> GPLHMKAVVPGPA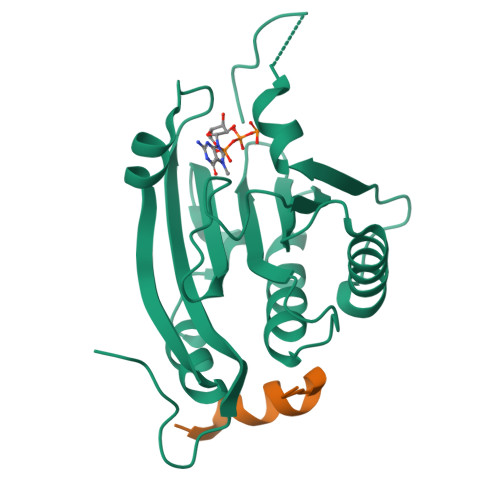EHPLQYNYTFWYSRRTPGRPTSSQSYEQNIKQIGTFASVEQFWRFYSHMVRPGDLTGHSDFHLFKEGIKPMWEDDANKNGGKWIIRLRKGLASRCWENLILAMLGEQFMVGEEICGAVVSVRFQEDIISIWNKTASDQATTARIRDTLRRVLNLPPNTIMEYKTHTDSIKMPGRLGPQRLLF;> RIIYDRKFLMECRNSPV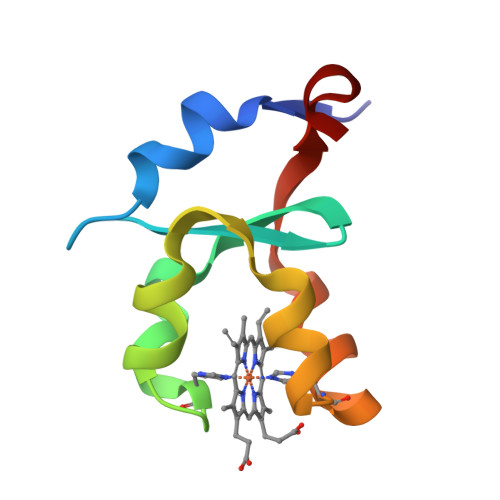> AVKYYTLEEIQKHNNSKSTWLILHYKVYDLTKFLEEHPGGEEVLREQAGGDATENFEDVGHSTDARELSKTFIIGELHPDDR> GCCCG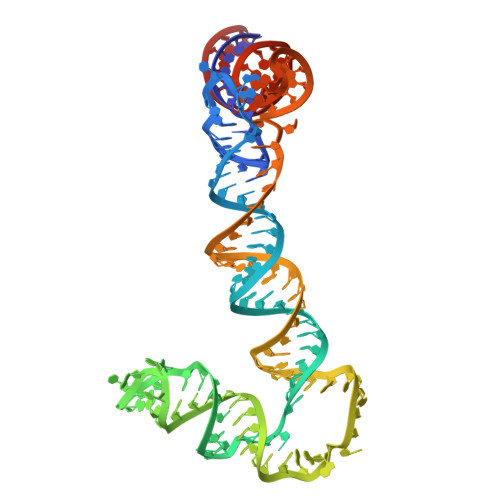GAUAGCUCAGUCGGUAGAGCAGCGGUAGCUGUUGAUCUGUGUGAAUCAGACUGCGACAGUUCGAGUUUGAAGCGAAAGCUAGCAACAGUAUCAACAGCUACCGCGGGUCCAGGGUUCAAGUCCCUGUUCGGGCGCCA IGF2 mRNA-binding protein 1 (IMP1) is a conserved RNA-binding protein that plays a key role in regulating cell motility, morphology and differentiation in the embryo, reviewed by Yisraeli. At the molecular level, IMP1 regulates the transport, translation and stability of a diverse ensemble of messenger RNAs (mRNAs). IMP1 contains six putative RNA-binding domains—two RNA-recognition motifs (RRMs) and four K-homology (KH) domains —which are conserved across species and found in pairs (RRM1RRM2, KH1KH2 and KH3KH4) that are closely spaced in the protein sequence. IMP1 function relies on the recognition of a diverse set of mRNA targets that is mediated by the combinatorial action of multiple RNA-binding domains.

In order to understand if and how the KH1 and KH2 domains also fold into a pseudo-dimer structure, we expressed an IMP1 construct that includes both domains (residues V194-N369) and determined the crystal structure. The structure shows that the KH1 and KH2 domains fold into an intra-molecular pseudo-dimer,, an arrangement found in a number of KH and RRM-containing proteins including the IMP1 KH3KH4 di-domain. Within the pseudo-dimer, the domains make contact through the two β1 strands, the inter-domain linker and the C-terminal α-helix of each domain (α3), burying a surface of ∼1200 Å2. Interestingly, many of the amino acids mediating the contacts between the two α3 helices (S254, C257, H265) are conserved in KH1KH2 across species but are very different in KH3KH4. In addition, KH1 α3 is longer than KH3 α3 and the linker between KH1 and KH2 is three amino acids shorter than that between KH3 and KH4, implying that the shorter KH1KH2 linker must span a longer distance to reach the amino-terminus of the second KH domain. In KH1KH2, after a sharp downward turn, the linker assumes a nearly linear conformation retracing the direction of the helix to reach the amino-terminal residue of KH2. The differences in the inter-domain interface result in a change in the angle between the two domains and, as a consequence, in a shorter distance (7–8Å) between the two RNA-binding grooves, as highlighted by the superimposition of the two structures. The structure also shows that the path between the RNA-binding grooves of KH1 and KH2 is positively charged, which may impact on the dynamics of RNA looping as discussed in our model below. In addition, the α3 of KH2 is extended by three turns. A plot of the RDCs measured in solution against those back-calculated from the structure reveals the high correlation (R2 = 0.97) between the two datasets, indicating that the crystal structure is highly representative of the protein conformation in solution.

> GAMVDIPLRLLVPTQYVGAIIGKEGATIRNITKQTQSKIDVHRKENAGAAEKAISVHSTPEGCSSACKMILEIMHKEAKDTKTADEVPLKILAHNNFVGRLIGKEGRNLKKVEQDTETKITISSLQDLTLYNPERTITVKGAIENCCRAEQEIMKKVREAYENDVAAMSLQSHLIPGLN>DIISVALKRHSTKAFDASKKLTPEQAEQIKTLLQYSPSSQNSQPWHFIVASTEEGKARVAKSAAGNYVFSERKMLDASHVVVFCAKTAMDDVWLKLVVDQEDADGRFATPEAKAANDKGRKFTADMHRKDLHDDAEWMAKQVYLNVGNFLLGVAALGLDAVPIEGFDAAILDAEFGLKEKGYTSLVVVPVGHHSVEDFNATLPKSRLPQNITLTEV[2x]

Escherichia coli NfsB has been studied extensively for its potential for cancer gene therapy by reducing the prodrug CB1954 to a cytotoxic derivative. The natural substrate of this flavoprotein enzyme is not known; however, it reduces a wide range of nitroaromatic compounds to hydroxylamines and also reduces quinones to quinols, with a bi-bi substituted (ping-pong) enzyme mechanism. The enzyme is a homodimer of two 24 kDa subunits with an extensive dimer interface. The two active sites are on opposite sides of the long central helix at the dimer interface, and the FMN is bound to residues from both monomers.

The most active mutant selected was T41Q/N71S/F124T. While the N71S is the only mutation at position 71 that enhances the activity of the protein for CB1954, the F124T mutation is not the most active mutation at position 124, and the T41Q mutation by itself reduces the activity of the protein for CB1954. The mutations together, therefore, show synergistic effects. In the triple mutant, the N71S mutation is the same as in the double mutant; position 41, however, is now a Gln, which is larger than the wild-type threonine and more polar than the leucine of the double mutant, while F124 has been replaced by threonine. In the structures of the free and nicotinate-bound triple mutant, the Q41 side chain forms a hydrogen bond to the T124 hydroxyl group, pulling the residue slightly closer than in the wild-type protein. In the structure without nicotinate, there is an acetate group in the active site, and Q41 forms a hydrogen bond to the carboxyl group of acetate so that this ligand is in a slightly different orientation than in the structure of the wild-type protein bound to acetate, determined previously, where the hydrogen bond cannot occur. The crystal structure of the T41Q/N71S/F124T mutant shows a hydrogen bond between Q41 and T124, explaining the co-operativity between these two residues. On replacing N71 with S71, in most of the structures of all the mutants, a water-mediated hydrogen bond to the FMN cofactor is found from the Oγ of S71 instead of the direct hydrogen bond from the NH2 of N71. In the triple mutant, two smaller bridges form between M127 and Y68 and between N67 and F123.>[2x]GKIILFEDVEFGGKKLELETSVSDLNVHGFNDIVSSIIVESGT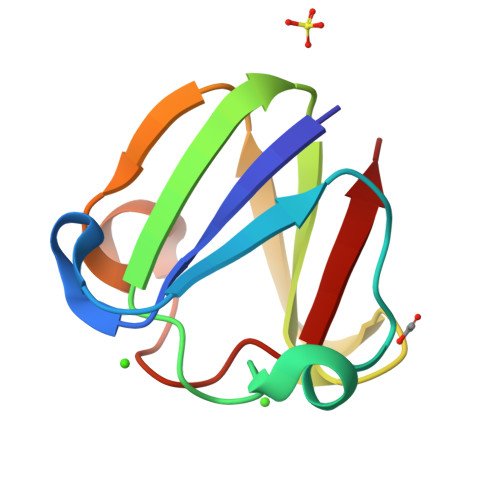WFVFDDEGFSGPSYKLTPGKYPNPGSWGGNDDELSSVKQQ>MRLCIPQVLLALFLSMLTAPGEGSRRRATQARDTTQPALLRLSDHLLANYKKGVRPVRDWRKPTTVSIDVIMYAILNVDEKNQVLTTYIWYRQYWTDEFLQWTPEDFDNVTKLSIPTDSIWVPDILINEFVDVGKSPNIPYVYVHHRGEVQNYKPLQLVTACSLDIYNFPFDVQNCSLTFTSWLHTIQDINITLWRSPEEVRSDKSIFINQGEWELLEVFPQFKEFSIDISNSYAEMKFYVIIRRRPLFYAVSLLLPSIFLMVVDIVGFCLPPDSGERVSFKITLLLGYSVFLIIVSDTLPATAIGTPLIGVYFVVCMALLVISLAETIFIVRLVHKQDLQRPVPDWLRHLVLDRIAWILCLGEQPMAHRPPA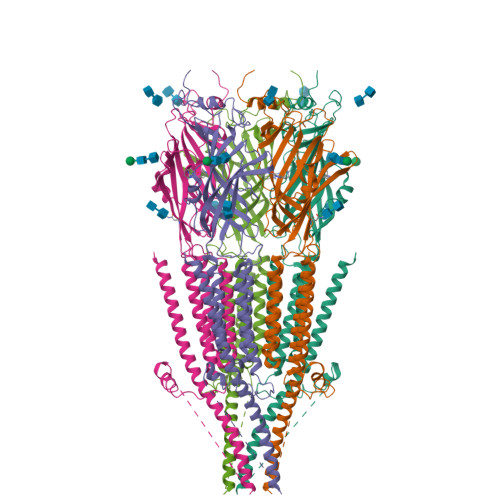TFQANKTDDCSGSDLLPAMGNHCSHVGGPQDLEKTPRGRGSPLPPPREASLAVRGLLQELSSIRHFLEKRDEMREVARDWLRVGYVLDRLLFRIYLLAVLAYSITLVTLWSIWHYS[5x]> MHHHHHHENLYFQSESLSWMQTGDTLALSGELDQDVLLP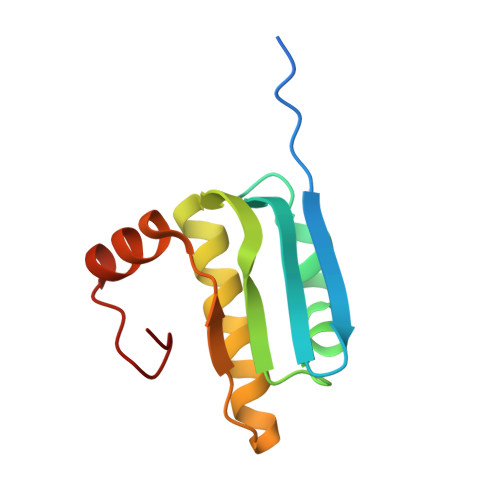LWEMREEAVKGITCIDLSRVSRVDTGGLALLLHLIDLAKKQGNNVTLQGVNDKVYTLAKLYNLPADVLPR> GHMSHASHDTGSTTVAGAACPAAGPHMMDPDLLADPFTGYGRLRERGPVVRGRFVDGTPVWFVTRYDDVRAVLRDPRFVNTPSPVPGEGGADPREGMMDLLNVPEPLRVYLLGSILDSDPPDHPRLRRLVTRAFAARRILGLRPGIERIADRLLAELPRREEEDGTVDLLEHFAYPLSITVICELVGIPATDLERWREWGGDLVSMRPERLRHSFPVMIDYCHRLIEQRRAALTDDLLSELIRAQDDDGGRLSDIETVTMILTLVLAGHETSAHLIGNGTAALLTHPGQWALLRKDPALLPRAVHELMRWCGSVHVARLRYATEDLELAG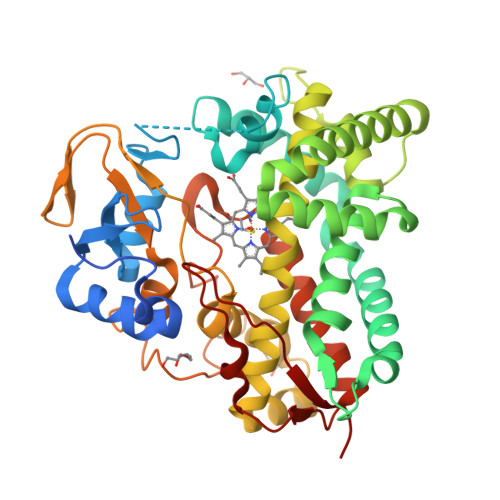TPVARGDAVQLVLVSANFDPRHYSDPDRLDITRHQEGQAENHVGFGHGIHYCLGATLARQEGEVALARLLETYPDLALADGDPEVRRARLPGSWRLDALRLRLRP> GAGCAGACCTGACGGAACTCA;> CCGTCA;> TCTGAGTT;> GGTCTGC

In this work, we exhaustively probe the ability of all 36 immobile HJ sequences to form DNA crystals in two different designed systems. Three separate self-assembling DNA crystal systems are described in this report: the “4 × 5” and “4 × 6” designs (collectively referred to as the 4 × N systems), and a third construct with a “scrambled” sequence variant of the 4 × 6 lattices. Self-assembly was mediated by three constituent oligonucleotides: (S1) containing four sequence repeats of either 5 or 6 bases; (S2) composed of 21 bases containing complementary regions to both (S1); and (S3) which forms the second junction crossover. The HJ serves as the fundamental component at the core of each unit, and the ultimate assembly of the full lattice is facilitated by the complementary 2-base sticky ends that tail each duplex.

Each asymmetric unit could be defined as either a HJ containing 10 and 11 bp on each arm, or as a 21-bp linear duplex. Seventeen of the 36 junctions successfully crystallized, a 47% success rate. Unlike the 4 × 5 motif, nearly all of the 4 × 6 junction sequences had a strong preference for crystallization in buffers containing ≥2.0 M salts (e.g., LiCl, Li2SO4, KCl, and NaCl), with the majority preferring slightly basic pH conditions in cacodylic acid. The average cell constants for the P32 crystals were a = b = 68.29 Å c = 55.68 Å.> MDIKVHFHDFSHVRIDCEESTFHELRDFFSFEADGYRFNPRFRYGNWDGRIRLLDYNRLLPFGLVGQIKKFCDNFGYKAWIDPQINEKEELSRKDFDEWLSKLEIYSGNKRIEPHWYQKDAVFEGLVNRRRILNLPTSAGRSLIQALLARYYLENYEGKILIIVPTTALTTQMADDFVDYRLFSHAMIKKIGGGASKDDKYKNDAPVVVGTWQTVVKQPKEWFSQFGMMMNDECHLATGKSISSIISGLNNCMFKFGLSGSLRDGKANIMQYVGMFGEIFKPVTTSKLMEDGQVTELKINSIFLRYPDEFTTKLKGKTYQEEIKIITGLSKRNKWIAK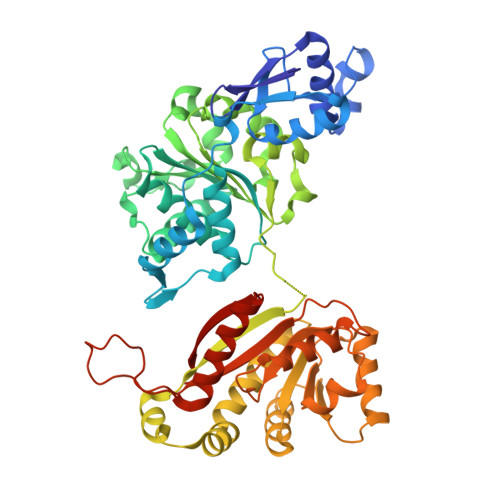LAIKLAQKDENAFVMFKHVSHGKAIFDLIKNEYDKVYYVSGEVDTETRNIMKTLAENGKGIIIVASYGVFSTGISVKNLHHVVLAHGVKSKIIVLQTIGRVLRKHGSKTIATVWDLIDDAGVKPKSANTKKKYVHLNYLLKHGIDRIQRYADEKFNYVMKTVNLLEHHHHHH1-[6-(2-CHLORO-4-METHYXYPHENOXY)-HEXYL]-IMIDAZOLE 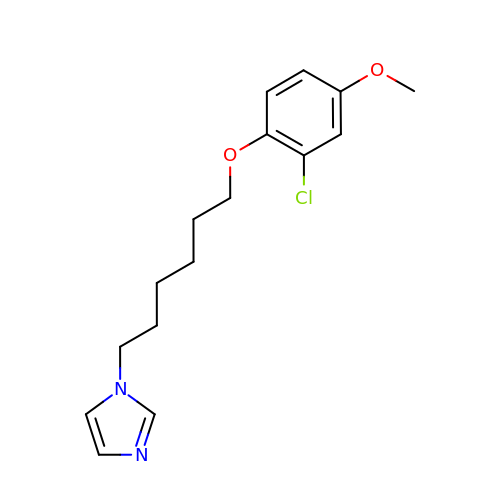| C16 H21 Cl N2 O2 | UKVVEWLDHJDSNJ-UHFFFAOYSA-N Aerobic RNR (class I) depends on the ferritin-like R2 subunit to generate a catalytic radical in an oxygen dependent reaction; the radical must be transferred back-and-forth with the catalytic R1 subunit, which performs the ribonucleotide reduction. Radical translocation between the subunits proceeds via reversible long-range proton-coupled electron transfer (PCET) in a transient R1-R2 complex. In a recently discovered active metal-free R2 subclass, denoted R2e, this tyrosine residue is post-translationally meta-hydroxylated to a 3,4-dihydroxyphenylalanine (DOPA) which serves as the radical-harboring residue. From an experimental point of view, R2e from Mesoplasma florum (MfR2) represents an attractive model to study active radical states in RNRs.

The catalytic radical can be chemically quenched by hydroxyurea, a known RNR radical scavenger used for decades as an antitumor drug proposed to inactivate R2 through PCET. Importantly, hydroxyurea causes a reversible inactivation of MfR2 as the enzyme can recover activity upon re-oxidation by NrdI. Thus, the protein is not permanently inactivated or damaged but resides in a radical-lost ground state. To ensure an accurate depiction of the radical-lost ground state of MfR2, we solved the crystal structure at 1.35 Å resolution of the protein chemically quenched by incubation with hydroxyurea before crystallization. This treatment abolished the 383-nm absorbance peak and rendered the protein colorless. The electron density map clearly shows the post-translational modification in the meta position of DOPAY126. The two oxygen-containing functional groups of DOPAY126 in the para and meta positions (denoted para-O and meta-O, respectively) form hydrogen bonds (H-bond) with D88. Strikingly, the meta-O is involved in a remarkably short interaction. Using END/RAPID error analysis, the O–O distance between DOPAY126 and D88 was calculated to 2.43 ± 0.04 Å, a length which could correspond to a low-barrier or single-well H-bond. In addition, DOPAY126 does not interact with any water, nor with K213 whose ε-ammonium group is facing away from DOPAY126.

>[2x]GHMASMAKIKNQYYNESVSPIEYAQQGFKGKMRSVNWNVVNDEKDLEVWNRITQNFWLPEKIPVSNDLTSWRTLTPEWQELITRTFTGLTLLDTIQATVGDVAQVPNSLTDHEQVIYTNFAFMVAVHARSYGSIFSTLCSSEQIEEAHEWVINTETLQERAKALIPYYVNDDPLKSKVAAALMPGFLLYGGFYLPFYLSARGKLPNTSDIIRLILRDKVIHNYYSGYKYQKKVAKLSPEKQAEMKEFVFKLLYELIDLEKAYLKELYEDFGLADDAIRFSVYNAGKFLQNLGYDSPFTEEETRIEPEIFTQLSARADENHDFFSGNGSSYIMGVSEETEDDDWEF> GSGSAKYTYRSLGRHLDFLRPGLRFGGSQSSKYTYYTVEVKIDTVNLPLYKDSRSLDPHVTGTFTIKNLTPVLDKVVTLFEGYVINYNQFPLCSLHWPAEETLDPYMAQRESDCSHWKRFGHFGSDNWSLTERNFGQYNH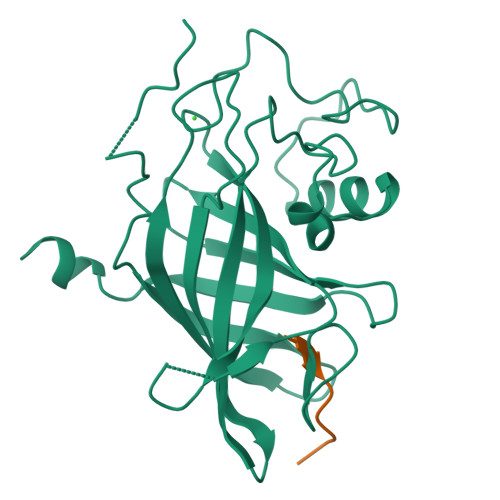ESAEFMNQRYIYLKWKERFLLDDEEQENLMLDDNHHLEGASFEGFYYVCLDQLTGSVEGYYYHPACELFQKLELVPTNCDALNT;> PFITSRPW> QRAEEE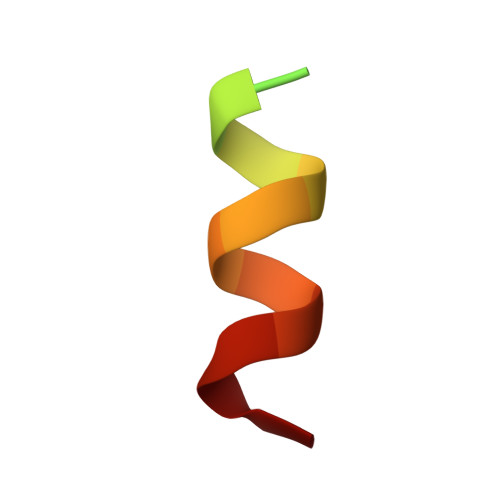DDDIKQLAAWAT> RALAAPLVHHHHHHALDENLYFQGALADVSRPPHARKTGGSSPETKYDQPPKCDISGKEAIS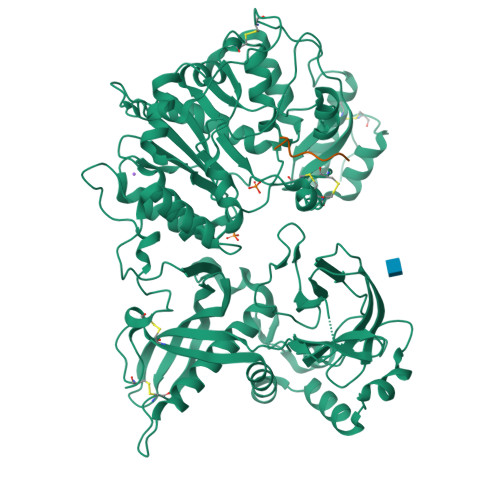ALSRAKSKHCRQEIGETYCRHKLGLLMPEKVTRFCPLEGKANKNVQWDEDSVEYMPANPVRIAFVLVVHGRASRQLQRMFKAIYHKDHFYYIHVDKRSNYLHRQVLQVSRQYSNVRVTPWRMATIWGGASLLSTYLQSMRDLLEMTDWPWDFFINLSAADYPIRTNDQLVAFLSRYRDMNFLKSHGRDNARFIRKQGLDRLFLECDAHMWRLGDRRIPEGIAVDGGSDWFLLNRRFVEYVTFSTDDLVTKMKQFYSYTLLPAESFFHTVLENSPHCDTMVDNNLRITNWNRKLGCKCQYKHIVDWCGCSPNDFKPQDFHRFQQTARPTFFARKFEAVVNQEIIGQLDYYLYGNYPAGTPGLRSYWENVYDEPDGIHSLSDVTLTLYHSFARLGLRRAETSLHTDGENSCRYYPMGHPASVHLYFLADRFQGFLIKHHATNLAVSKLETLETWVMPKKVFKIASPPSDFGRLQFSEVGTDWDAKERLFRNFGGLLGPMDEPVGMQKWGKGPNVTVTVIWVDPVNVIAATYDILIESTAEFTHYKPPLNLPLRPGVWTVKILHHWVPVAETKFLVAPLTFSNRQPIKPEEALKLHNGPLRNAYMEQSFQSLNPVLSLPINPAQVEQARRNAASTGTALEGWLDSLVGGMWTAMDICATGPTACPVMQTCSQTAWSSFSPDPKSELGAVKPDGRLR;> QEEEGSGGGQGG>MEGVQEILSRAGIFQGVDPTAVNNLIQDMETVRFPRGATIFDEGEPGDRLYIITSGKVKLARHAPDGRENLLTIMGPSDMFGELSIFDPGPRTSSAVCVTEVHAATMNSDMLRNWVADHPAIAEQLLRVLARRLRRTNASLADLIFTDVPGRVAKTLLQLANRFGTQEAGALRVNHDLTQ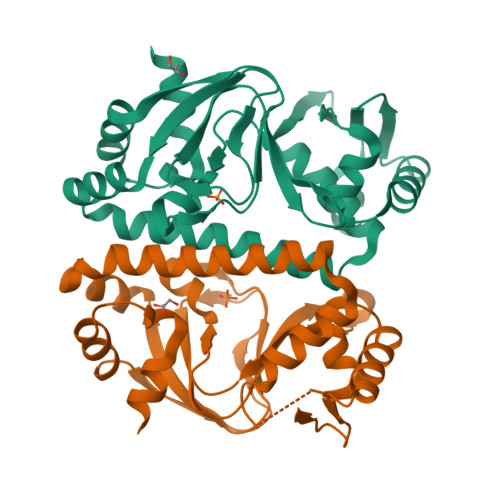EEIAQLVGASRETVNKALATFAHRGWIRLEGKSVLIVDTEHLARRAR[2x]3'-fluoro-4'-(trifluoromethyl)biphenyl-4-sulfonamide 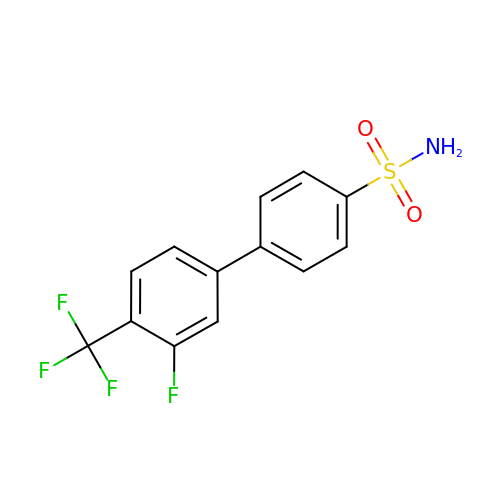| C13 H9 F4 N O2 S | UEPKMFLFRNDVAW-UHFFFAOYSA-N>[4x]MGDPEEYEDQLEETLEQKEYEDHDSVSIPMEEAEGDTIQEEEAEARVNQLTDTDYHTTSQHPETHKVCVQLRELVMDEKNQEIQWMETARWVGLEENLGKDGIWGRPHLPYLNFWSLLELQKAFAKGTVLLDLPGKSLAEVANQLLDRFTFEGQIQPDDQDNLLRVLLLKHSHASDMEALGGVKPVVVTHSGDPSEPLLPQHPSLETELFCEQGEGSTRGHAPEILGKSPQDWEATLVLVGCARFLKRPVLGFVRLKEPMEPEPKPEGSEEPAVPVRFLIVLLGPEGPNINYTQLGRAAATLMSERVFWNDAYLAQSKETLVQSLEGFLDC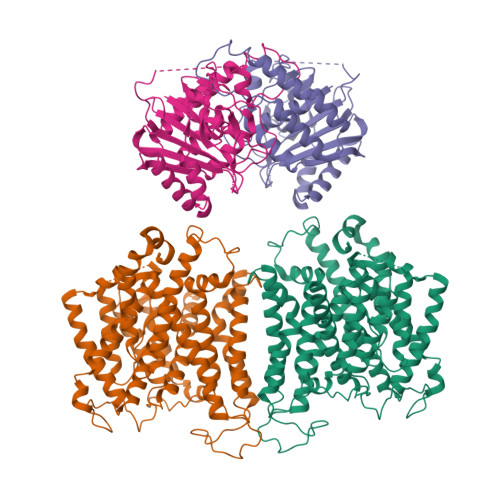SLVLPPLDAPSEKALLSLVPVQKELLRRRYLPSPAKPDPSIFKDLDVKKGPGDTPEDPLQRTGKLFGGLVRDIRRRYPRYLSDITDALSPQVLSAIIFIYFAALTPAITFGGLLGDKTENMIGVSELLLSTALQGIIFSLLGAQPLLVLGFSGPLLVFEEAFYSFCQTNNLEYIVGRVWIGFWLILLVVLVVAFEGSFLVRFISRYTQEIFSFLISLIFIYETFYKLVTIFQDHPLQKNYDHDVLTTPKPQAALPNTALLSLVLMAGTFFLAMMLRKFKNSSYFPGKLRRIIGDFGVPISILIMVMVDALIQDTYTQKLSVPEGLSVSNPTERDWLIHPLGIRVEFPIWMMFASALPALLVFILIFLESQITTLIISKPERKMVKGSGFHLDLLLIIGMGGVGAIFGMPWLSATTVRTVTHANALTVMSKDSTPGAVSQIQGVKEQRISGLLVAVLVGVSILMGPVLRHIPLAVLFGIFLYMGVTSLSGIQLFDRVLLLLKPRKYYPEVPYARRVKTWRMHLFTITQIVCLVVLWVVRSIKQISLALPFILILTVPLRRFLLPFIFRDMELKLLDADDVKLNLDEQNGQDEYDEVAMPV> PAVEVRLDKW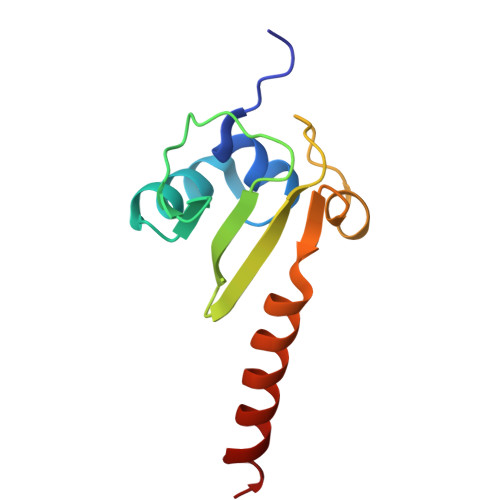LWAARFYKTRALAREMIEGGKVHYNGQRSKPSKIVELNATLTLRQGNDERTVIVKAITEQRRPASEAALLYEETAESVEKREKMALARKLNALT> MQFFKTLAALVSCISFVLAYVAQDVHVSFPSTAGKSRVMIGKVEPRIGIDETVPTTITVEDPNEVIQVNFAIESTNKPFQNTLLIGLPNKNLEMAFEPEIKDNGKLSMYKYRIDLAKLDAALLQEASRSPEPIKATLILASSTAKPKENLFREILQLNLNFDVDHSDSSLVDKFGIKPEIHHIFHAEPKRVAKPIAVIFVLIIFITILSLIVTWLNSCAAAFNNIPTGVTAVYFLGFIATIVGFE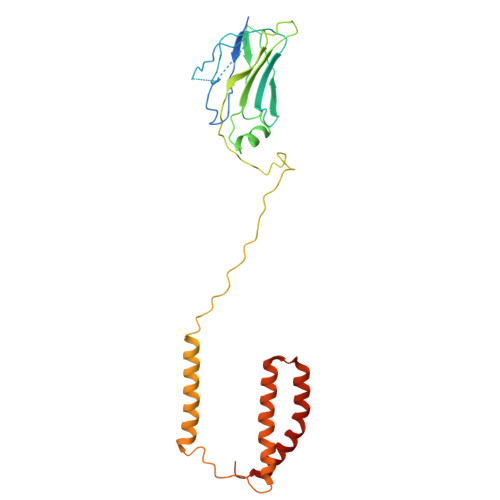VIFARYYLGTSIFETLFSSLYLGAPGLLTSTKFLRSFGQTI>GARRRRTRCRRCRACVRTECGDCHFCRDMKKFGGPGRMKQSCLLRQ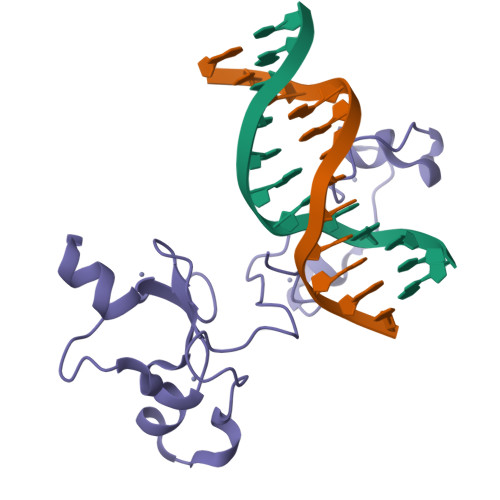CTAPVLPHTAVCLLCGEAGKEDTVEGEEEKFGLSLMECTICNEIVHPGCLKMGKAEGVINAEIPNCWECPRCTQEGR[4x]>[2x]MTPNKEDYLKIIYELSERDEKISNKQIAEKMSVSAPAVSEMVKKLLLEDLVLKDKQAGYLLTKKGQILASSLYRKHRLIEVFLMNHLNYTADEIHEEAEVLEHTVSDVFVERLDKFLNYPK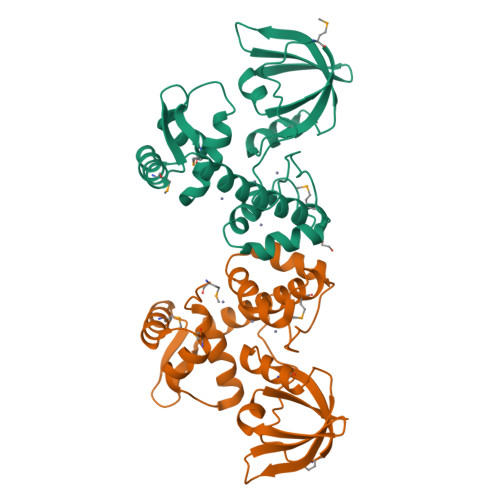VCPHGGTIPQHGQPLVERYRTTLKGVTEMGVYLLKRVQDNFQLLKYMEQHHLKIGDELRLLEYDAFAGAYTIEKDGEQLQVTSAVASQIYIEKK The cellular role of DNPH1 is to remove hydroxymethyl deoxyuridine monophosphate (hmdUMP) from the nucleotide pool. Hydrolysis generates deoxyribose monophosphate (dRP) and hydroxymethyl uracil (hmU) products. Glycosidic bond cleavage is driven by a conserved catalytic triad and proceeds via a two-step mechanism involving formation and subsequent disruption of a covalent glycosyl-enzyme intermediate. Each DNPH1 monomer adopts a Rossmann-like fold consisting of five core β-strands surrounded by five major α-helices.

To visualise the trapping of the glycosyl-enzyme intermediate, we employed a crystallisation construct harbouring a single E55Q point mutation. Purified DNPH1E55Q protein was co-crystallised with hmdUMP and the structure solved in space group P212121 at 1.65 Å resolution using the DNPH1E104Q structure for molecular replacement. In the crystal structure a biologically active homodimer comprises the asymmetric unit, and both active sites contain a trapped glycosyl-enzyme intermediate with deoxyribose monophosphate (dRP) covalently fused to E104. However, in both chains, the dRP:E104 moiety adopts two distinct, alternative conformations, one of which permits an additional interaction between the constituent sugar and surrounding sidechains. The base of the substrate has been cleaved and is no longer visible, but has been largely replaced by a well-defined water network. This network is stabilised in part by E55Q, which is now presented into the active site through reorganisation of the helical element harbouring the LTEHV motif. Consequently, H56 tucks away below the anomeric carbon. Remarkably, E55Q appears to be ideally positioned although, due to the mutation, chemically unable to activate one of the bound waters for nucleophilic attack at the anomeric carbon, in agreement with activity assays. Crucially, the conserved catalytic aspartate (D80) is too far away to perform this activation, and the active site arrangement indicates that this is also the case in the wild-type enzyme. In this dominant arrangement, H56 electrostatically drives the dRP 3′ hydroxyl group to form a hydrogen bond with the remaining sidechain carbonyl oxygen of E104.

>[2x]GSMGRPALYFCGSIRGGREDRTLYERIVSRLRRFGTVLTQHVAAAELGARGEEAAGGDRLIHEQDLEWLQQADVVVAEVTQPSLGVGYELGRAVAFNKRILCLFRPQSGRVLSAMIRGAADGSRFQVWDYEEGEVEALLDRYFEADP>GPGSEFELPLPEGWEEARDFDGKVY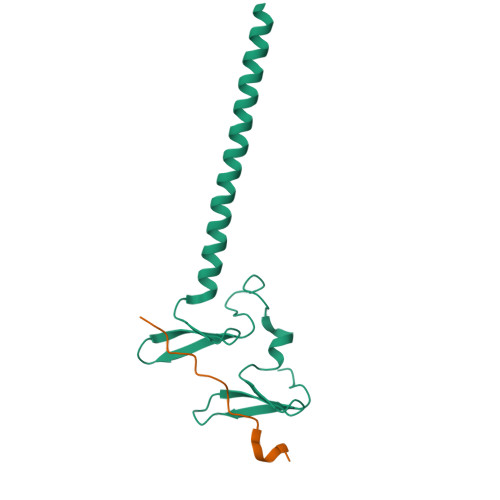YIDHRNRTTSWIDPRDRYTKPLTFADCISDELPLGWEEAYDPQVGDYFIDHNTKTTQIEDPRVQWRREQEHMLKDYLVVAQEALSAQKEIYQVKQQRLELAQQEYQQLH[2x];>GPGSVAEAPSYQGPPPPYPKHLLHQNPS[2x]> MNNSVGSTHNVTILGSGETTVVLSHGYGTDQSVWKLFVPHLVDDYRVLLYDNMGAGTTNPDYFDFERYSSLEGYSYDLIAILDEFHVSKCIFVGHSMSAMAAAVASIFRPDLFHKLIMISPSPRLANAEDYYGGLEQKEIDEVVGSMEENYRSMALGSAPLLLA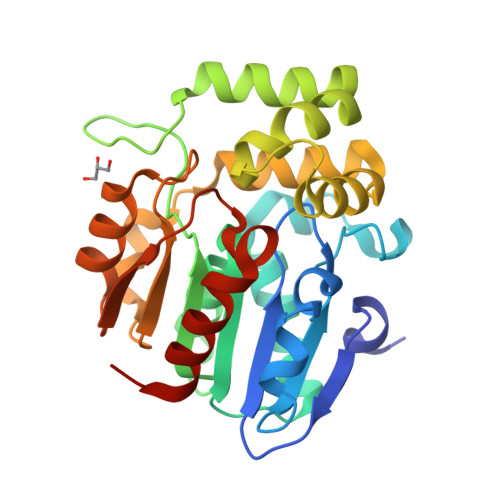CDLESAAVQEYCRTLFNMRPDISCCMARMIFGLDLRPYLCHVTVPCHILQSSNDVMVPVAVVEYLSKNLGGPSVVEVMPTEGHLPHLSAPEVTIPVVLRHIRHDIADQ> XQNGF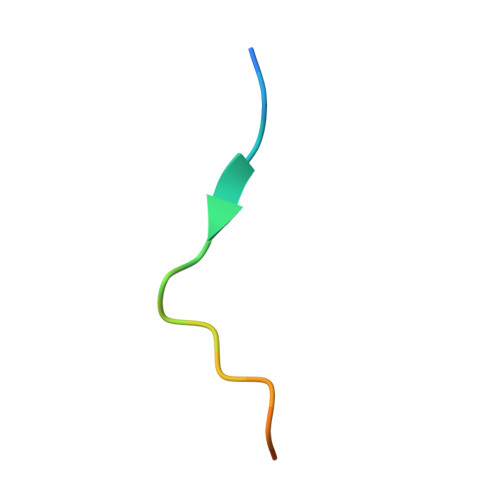DNPNYQPQENMQA> GPVEDAVTAAIGRVADTVGTGPTNSEAIPALTAAETGHTSQVVPGDTMQTRHVKNYHSRSESTVENFLCRSACVYFTEYKNSGSKRYAEWVVTTRQAAQLRRKLEFFTYIRFDLELTFVITSTQQPSTTQNQDAQILTHQIMYVPPGGPVPDKVDSYVWQTSTNPSVFWTEGNAPPRMSIPFLSIGNAYSNFYDGWSDFSRDGVYGINTLNSMGTLYARHVNTGGTGPIKSTIRIYFKPKHVKAWIPRPPRLCQYEKAKNVNFQPSGVTTTRQSITAMTNTGAF;> SPTVEECGYSDRVRSITLGNSTITTQECANVVV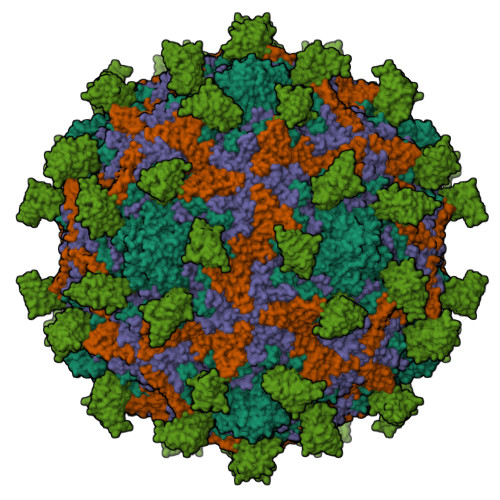GYGVWPDYLKDNEATAEDQPTQPDVATCRFYTLDSVQWQKTSPGWWWKLPDALSNLGLFGQNMQYHYLGRTGYTIHVQCNASKFHQGCLLVVCVPEAEMGCATLDNTPSSAELLGGDAAKEFAGEPIASGSNKLVQRVVYNAGMGIGVGNLTIFPHQWINLRTNNSATIVMPYTNSVPMDNMFRHNNVTLMVIPFVPLDYCPGSTTYVPITVTIAPMNAEYNGLRLAGHQ;> GLPTMNTPGSCQFLTSDDFQSPSAMPQYDVTPEMRIPGEVKNLMEIAEVDSVVPVQNVGEKVNSMEAYQIPVRSNEGSGTQVFGFPLQPGYSSVFSRTLLGEILNYYTHWSGSIKLTFMFCGSAMATGKFLLAYSPLGAGAPTKRVDAMLGTHVVWDVGLQSSCVLCIPWISQTHYRYVASDECTAGGFITCWYQTNIVVPADAQSSCYIMCFVSACNDFSVRLLKDTPFISQENFFQ;> GAQVSTQKTGAHETGLNASGNSIIHYTNINYYKDAASNSATRQDFAQDPGKFTEPVKDIMIKSLPALN;> MSITTPEEMIEKAKGETAYLPCKFTLSPEDQGPLDIEWLISPADNQKVDQVIILYSGDKIYDDYYPDLKGRVHFTSNDLKSGDASINVTNLQLSDIGTYQCKVKKAPGVANKKIHLVVLVKPSGARCYVDGSEEIGSDFKIKCEPKEGSLPLQYEWQKLSDSQKMPTSWLAEMTSSVISVKNASSEYSGTYSCTVRNRVGSDQCLLRLNVVPPSNKALE> MGFSADHSQIAQTKDTMFTGYLDPVQAKDYFAEAEKTSIVQRVAQKIPMGATGIVIPHWTGDVSAQWIGEGDMKPITKGNMTKRDVHPAKIATIFVASAETVRANPANYLGTMRTKVATAIAMAFDNAALHGTNAPSAFQGYLDQSNKTQSISPNAYQGLGVSGLTKLVTDGKKWTHTLLDDTVEPVLNGSVDANGRPLFVESTYESLTTPFREGRILGRPTILSDHVAEGDVVGYAGDFSQIIWGQVGGLSFDVTDQATLNLGSQESPNFVSLWQHNLVAVRVEAEYGLLINDVNAFVKLTFDPVLTTYALDLDGASAGNFTLSLDGKTSANIAYNASTAT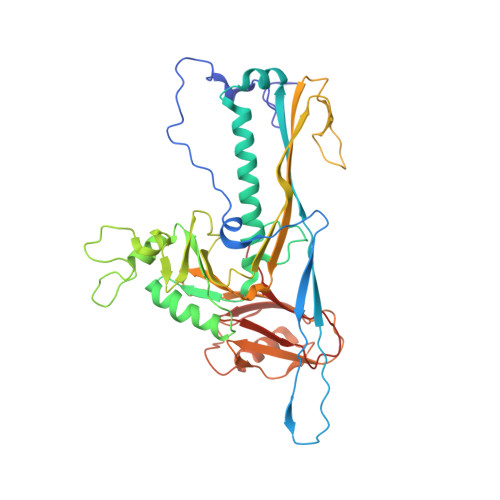VKSAIVAIDDGVSADDVTVTGSAGDYTITVPGTLTADFSGLTDGEGASISVVSVG7-({[3-(4-methylpyridin-3-yl)propyl]amino}methyl)quinolin-2-amine 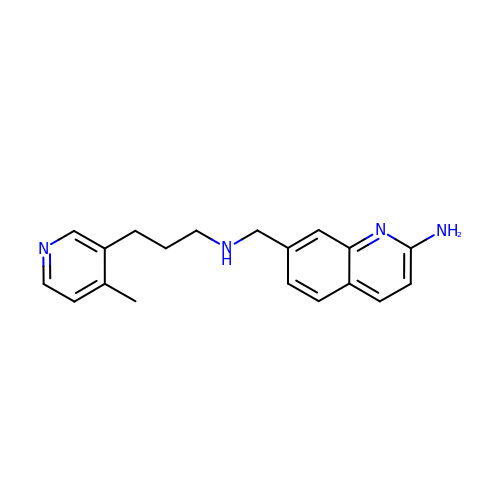| C19 H22 N4 | DURWIDBNTFVYBY-UHFFFAOYSA-N> MSQRLDILKALTAHLEQITIANGYAYDLKGKVYRGRDRFGADFTSRLPIVSILEAKATDYGSFANEEQTVRMDDWVLLVQGWVKDDPRNPTDPAYELLAEVEKRLAMLVAKDEQGQPMYPALYRLGGKIAKL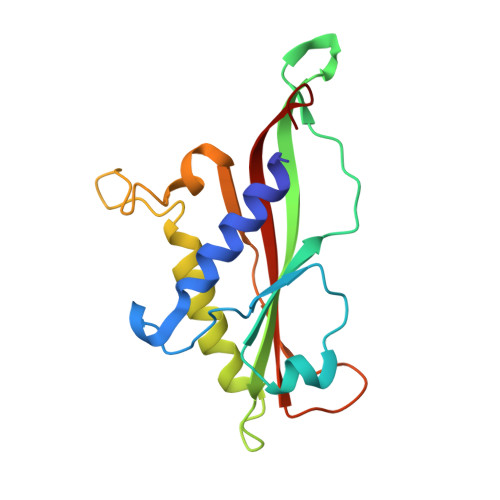TLAQPVVRPPEDGLSDTAFFFLPVRVGLKVDIRNP> ANKNMKILIVDDFSTMRRIVKNLLRDLGFNNTQEADDGLTALPMLKKGDFDFVVTDWNMPGMQGI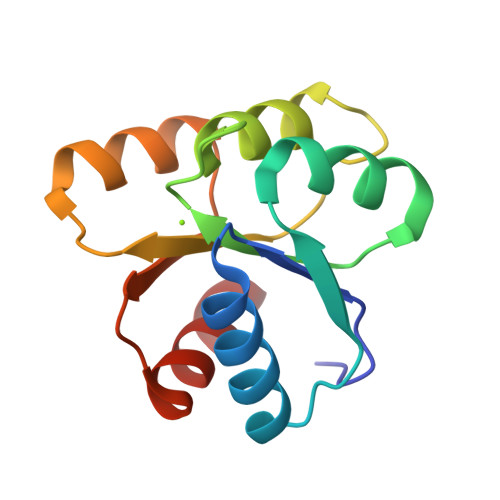DLLKNIRADEELKHLPVLMITAEAKREQIIEAAQAGVNGYIVKPFTAATLKEKLDKIFE> TIQPGTGYNNGYFYSYWNDGHGGVTYTNGPGGQFSVNWSNSGDFVGGKGWQ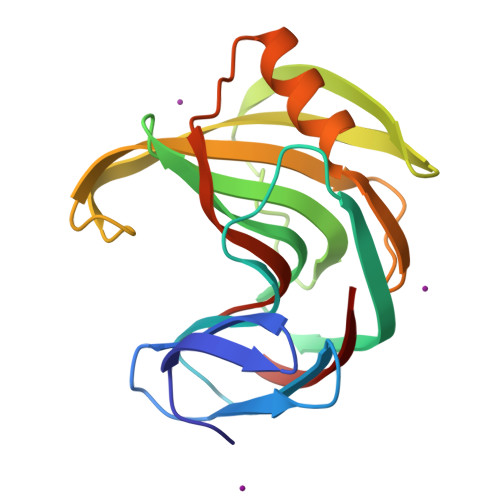PGTKNKVINFSGSYNPNGNSYLSVYGWSRNPLIEYYIVENFGTYNPSTGATKLGEVTSDGSVYDIYRTQRVNQPSIIGTATFYQYWSVRRNHRSSGSVNTANHFNAWAQQGLTLGTMDYQIVAVQGYFSSGSASITVS> MPPGVDCPMEFWTKEESQSVVVDFLLPTGVYLNFPVSRNANLSTIKQVLWHRAQYEPLFHMLSDPEAYVFTCVNQTAEQQELEDEQRRLCDIQPFLPVLRLVAREENLYFQGGDRVKKLINSQISLLIGKGLHEFDSLRDPEVNDFRTKMRQFCEEAAAHRQQLGWVEWLQYSFPLQLEPSARGWRAGLLRVSNRALLVNVKFEGSEESFTFQVSTKDMPLALMACALRKKATVFRQPLVEQPEEYALQVNGRHEYLYGNYPLCHFQYICSCLHSGLTPHLTMVHSSSILAMRDEQSNPAPQVQKPRAKPPPIPAKKPSSVSLWSLEQPFSIELIEGRKVNADERMKLVVQAGLFHGNEMLCKTVSSSEVNVCSEPVWKQRLEFDISVCDLPRMARLCFALYAVVEKAKKARSTKKKSKKADCPIAWANLM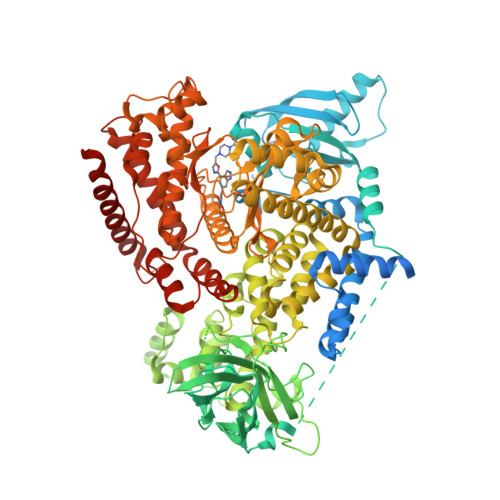LFDYKDQLKTGERCLYMWPSVPDEKGELLNPAGTVRGNPNTESAAALVIYLPEVAPHPVYFPALEKILELGRHGERGRITEEEQLQLREILERRGSGELYEHEKDLVWKMRHEVQEHFPEALARLLLVTKWNKHEDVAQMLYLLCSWPELPVLSALELLDFSFPDCYVGSFAIKSLRKLTDDELFQYLLQLVQVLKYESYLDCELTKFLLGRALANRKIGHFLFWHLRSEMHVPSVALRFGLIMEAYCRGSTHHMKVLMKQGEALSKLKALNDFVKVSSQKTTKPQTKEMMHMCMRQETYMEALSHLQSPLDPSTLLEEVCVEQCTFMDSKMKPLWIMYSSEEAGSAGNVGIIFKNGDDLRQDMLTLQMIQLMDVLWKQEGLDLRMTPYGCLPTGDRTGLIEVVLHSDTIANIQLNKSNMAATAAFNKDALLNWLKSKNPGEALDRAIEEFTLSCAGYCVATYVLGIGDRHSDNIMIRESGQLFHIDFGHFLGNFKTKFGINRERVPFILTYDFVHVIQQGKTNNSEKFERFRGYCERAYTILRRHGLLFLHLFALMRAAGLPELSCSKDIQYLKDSLALGKTEEEALKHFRVKFNEALRESWKTKVNWLAHNVSKDNRQ> MLRPTCPVAKNLTSFATKGTMRGGIPRIYYTWMKPGSATRRRFEKMRNPFVNLETGTSLYFRDTRDSAEAVAHAADSKGLKGMDNGVDLYNEYKIVPDLYPEGFQWKHKLNTEYNQWRSNTWLTPELIPQEHRGRFLCNFQLNIVAYDMRVVKFSPKDHRQWIYCVLYVGTGKGIAGFGRAVAPSTQEARNEAIREAFSNIIAVDLEQEGPMYPVRINADGARVLLYPARRIIANFRVADILCAFGFQNAGCKINLKASNNPKAPTHTVEGVFEAVKALRSVSEIAASRGKVPHSLVYNIYPYLEEMRRRKGMMAMHPPGKDGIFMPNRVVDNRMPDHLKKGYYDDVYWKDFFAGSKEQLNEPKMGLRGDELRAQLEESQGRTAKRSNRR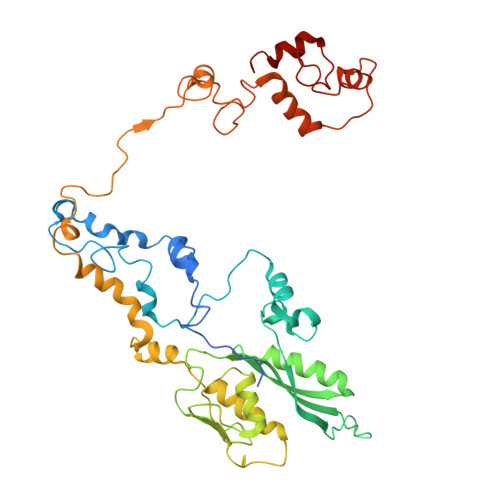TLDDVLRRLGKTSRDLGALQVVNPRLDAKLPTHMKRNYLLH>[2x]TYTTRQIGAKNTLEYKVYIEKDGKPVSAFHDIPLYADKENNIFNMVVEIPRWTNAKLEITKEETLNP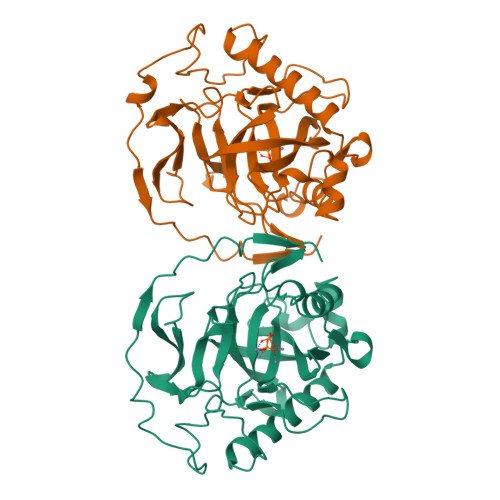IIQDTAKGKLRFVRNCFPHHGYIHNYGAFPQTWEDPNVSHPETKAVGDNDPIDVLEIGETIAYTGQVKQVKALGIMALLDEGETDWKVIAIDINDPLAPKLNDIEDVEKYFPGLLRATNEWFRIYKIPDGKPENQFAFSGEAKNKKYALDIIKETHDSWKQLIAGKSSDSKGIDLTNVTLPDTPTYSKAASDAIPPASPKADAPIDKSIDKWFFISGSV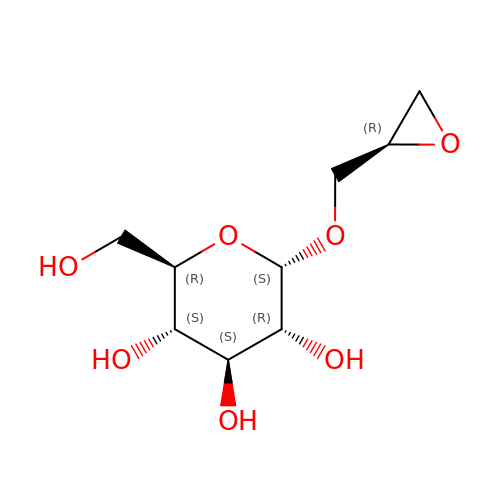(2R)-oxiran-2-ylmethyl alpha-D-glucopyranoside | C9 H16 O7 | NXJZWOCFSMYDAS-NZJLWHDDSA-N>[4x]MEIPVIEPLFTKVTEDIPGAEGPVFDKNGDFYIVAPAVEVNGKPAGEILRIDLKTGKKTVICKPEVNGYGGIPAGCQCDRDANQLFVADMRLGLL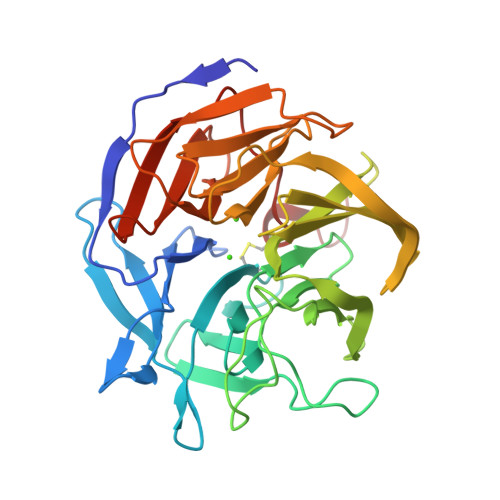VVQTDGTFEEIAKKDSEGRRMQGCNDCAFDYEGNLWITAPAGEVAPADATASMQEKFGSIYCFTTDGQMIQVDTAFQFPNGIAVRHMNDGRPYQLIVAEMPTKKLWSYDIKGPAKIENKKVWGHIPGTHEGGADGMDFDEDNNLLVANWGSSHIEVFGPDGGQPKMRIRCPFEKPSNLHFKPQTKTIFVTEHENNAVWKFEWQRNGKKQYCETLKFGIF> ERAGPVTWVMMIACVVVFIAMQILGDQEVMLWLAWPFDPTLKFEFARYFTHALMHFSLMHILFNLLWWWYLGGAVEKRLGSGKLIVITLISALLSGYVQQKFSGPWFGGLSGVVYALMGYVWL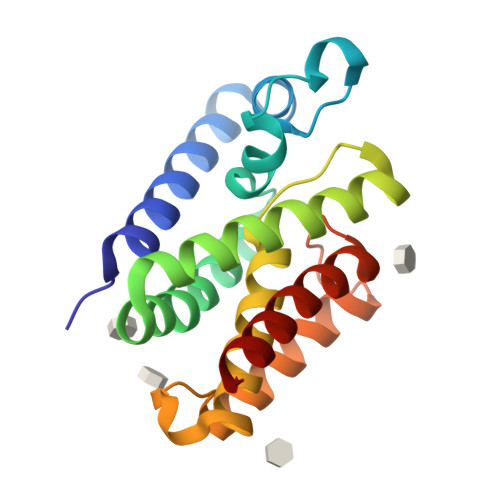RGERDPQSGIYLQRGLIIFALIWIVAGWFDLFGMSMANGAHIAGLAVGLAMAFVDSL>GSHMLEQKK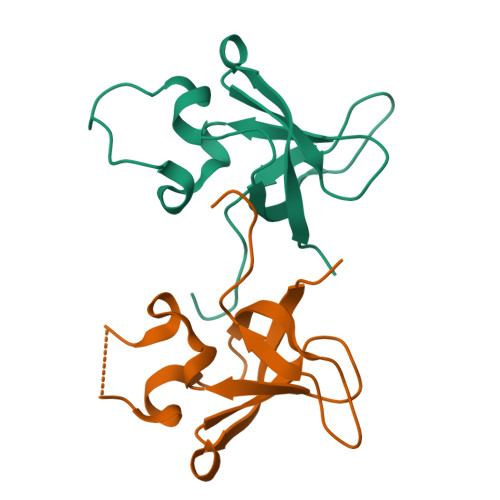ANIYKGKITRIEPSLEAAFVDYGAERHGFLPLKEIAREYFPANYSAHGRPNIKDVLREGQEVIVQIDKEERGNKGAALTTFISLAGS[2x]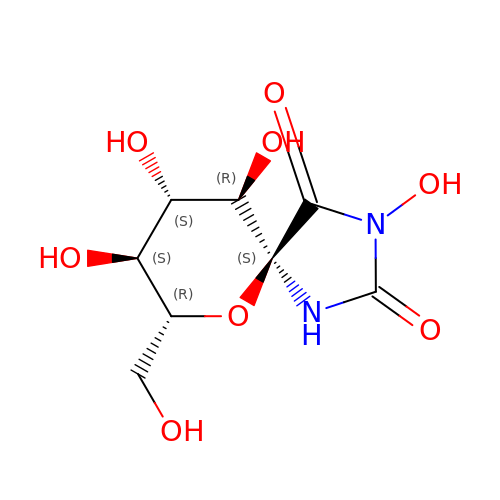(5S,7R,8S,9S,10R)-3,8,9,10-tetrahydroxy-7-(hydroxymethyl)-6-oxa-1,3-diazaspiro[4.5]decane-2,4-dione | C8 H12 N2 O8 | IHDZZZHACPJCFJ-WWHASAIZSA-N> TCTGT;> CGGACAGCACCTCGCA;> ACACCG;>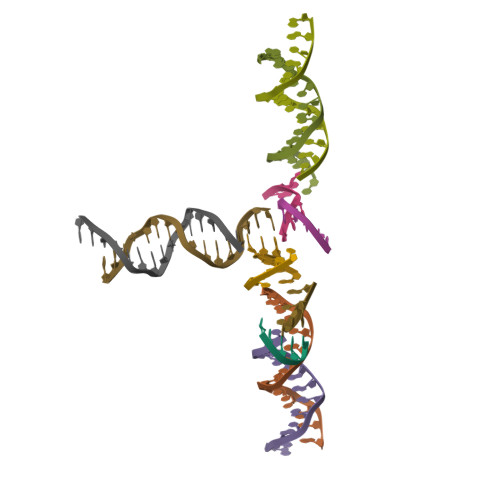 GATGCGAGGTGCTGT>MSQVILDLQLACEDNSGLPEESQFQTWLNAVIPQFQEESEVTIRVVDTAESHSLNLTYRGKDKPTNVLSFPFEVPPGMEMSLLGDLVICRQVVEKEAQEQGKPLEAHWAHMVVHGSLHLLGYDHIEDDEAEEMEALETEIMLALGYEDPYIAE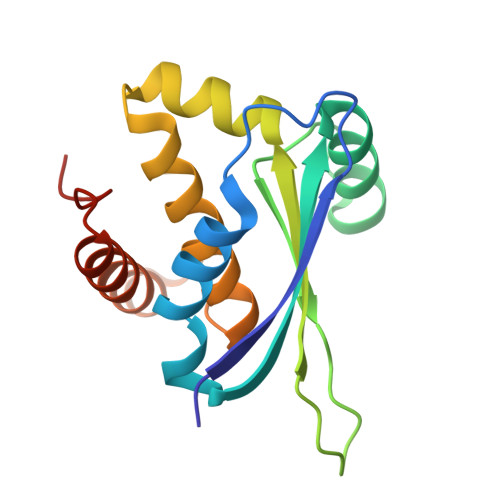KE[4x]> SV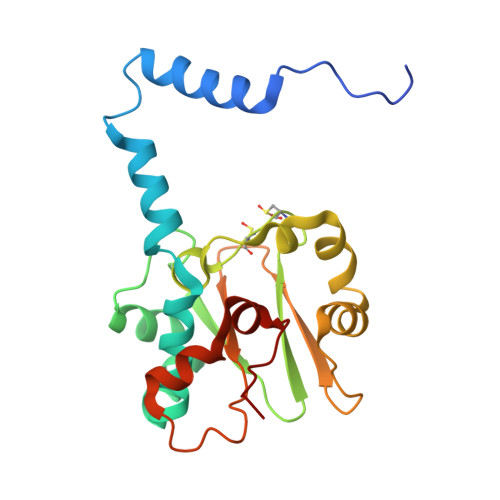TIDHTTENAAPAQAPVSDRAWALFRALDGKGLVPDGYVEGWKKTFEEDFSPRRGAELVARAWTDPEFRQLLLTDGTAAVAQYGYLGPNGEYIVAVEDTPTLKNVIVCSLCSCTAWPILGLPPTWYKSFEYRARVVREPRKVLSEMGTEIASDIEIRVYDTTAETRYMVLPQRPAGTEGWSQEQLQEIVTKDCLIGVAIPQVPTV> XSEEALPAS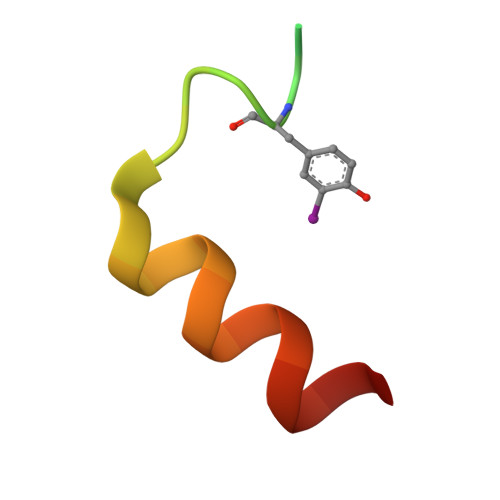GKSKYEAMDFDSLLKEAQQSLH3-[2-(2-amino-4-methylquinolin-7-yl)ethyl]-5-[(methylamino)methyl]benzonitrile 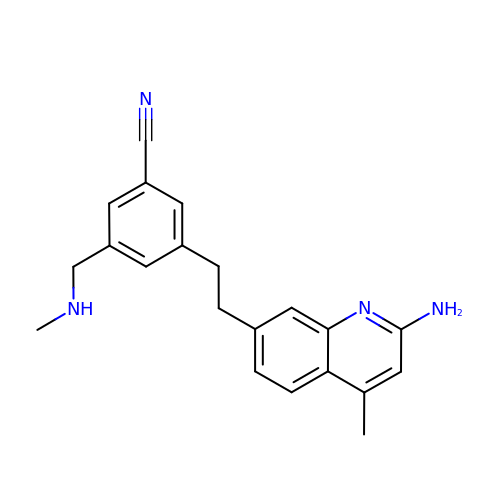| C21 H22 N4 | RWCOIXDPXHFMEG-UHFFFAOYSA-N> GIHFGNLARVRHIITYSLSPFEQR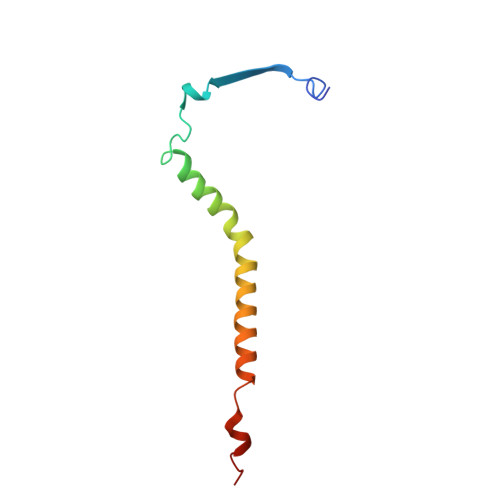AIPNIFSDALPNVWRRFSSQVFKVAPPFLGAYLLYSWGTQEFERLKRKNPADYENDQ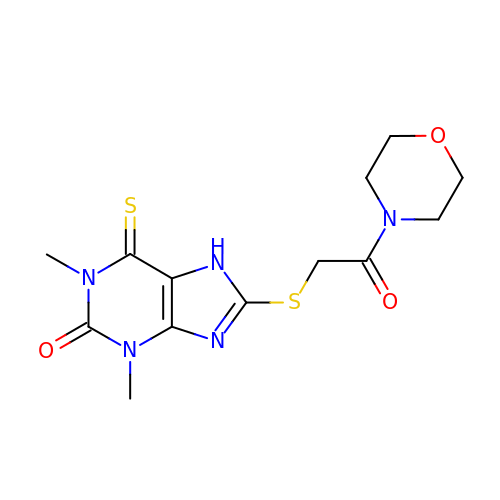1,3-dimethyl-8-{[2-(morpholin-4-yl)-2-oxoethyl]sulfanyl}-6-sulfanylidene-1,3,6,7-tetrahydro-2H-purin-2-one | C13 H17 N5 O3 S2 | KRPVEFPMIUNCJW-UHFFFAOYSA-N> GSHMASNVLALDTSQRIRIGLRKGEDLFEISYTGEKKHAEILPVVVKKLLDELDLKVKDLDVVGVGIGPGGLTGLRVGIATVVGLVSPYDIPVAPLNSFEMTAKSCPADGVVLVARRARKGYHYCAVYLKDKGLNPLKEPSVVSDEELEEITKEFSPKIVLKDDLLISPAVLVEESERLFREKKTIHYYEIEPLYLQKSIAELNWEKKKRG;> EGRMRVLGIETSCDETAVAVLDDGKNVVVNFTVSQIEVHQKFGGVVPEVAARHHLKNLPILLKKAFEKVPPETVDVVAATYGPGLIGALLVGLSAAKGLAISLEKPFVGVNHVEAHVQAVFLANPDLKPPLVVLMVSGGHTQLMKVDEDYSMEVLGETLDDSAGEAFDKVARLLGLGYPGGPVIDRVAKKGDPEKYSFPRPMLDDDSYNFSFAGLKTSVLYFLQREKGYKVEDVAASFQKAVVDILVEKTFRLARNLGIRKIAFVGGVAA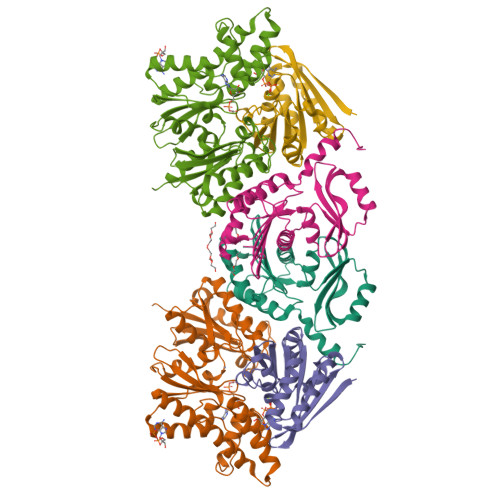NSMLREEVRKRAERWNYEVFFPPLELCTDNALMVAKAGYEKAKRGMFSPLSLNADPNLNV;> ASRHLRFENLTEEQLKRLAKILTENLKGGEVVILSGNLGAGKTTFVKGMIRAIGLDEKMVKSPTFTLMNVYPGLKTIYHLDLYRLQDTDFLSLDVEDILEDEDGIMVVEWGDLFDGFWPEDSIKVKIEIADESHRNVEILIPEEVNFLVEKIERYRKELQNT> SVPAEGAFTEDFQGLRAEVETISKELELLDRELCQLLLEGLEGVLRDQLALRALEEALEQGQSLGPVEPLDGPAGAVLECLVLSSGMLVPELAIPVVYLLGALTMLSETQHKLLAEALES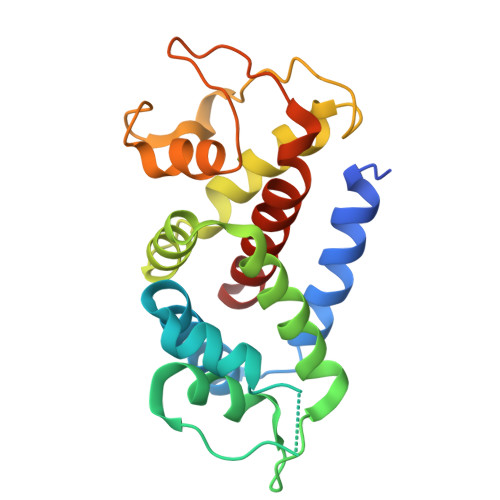QTLLGPLELVGSLLEQSAPWQERSTMSLPPGLLGNSWGEGAPAWVLLDECGLELGEDTPHVCWEPQAQGRMCALYASLALLSGLSQEPH> MTMPNGSGGLDPGAWLSHWVNQADLSSLAGRTEDEVRAYFENLVQADSGWGDASNTFFNLILGGFQNLSEFVTLIVQAVTGAPGGLTDLQAFLTERWGDLADAFQAVANLIDAIAGEVGSSLADAIAKLATFLTELSPLNAGMLFGLIGTNHLPLLSVSHIANINPELLVNAGFDSDVSVVDNPYWDWDGTVGRTAPLGAVKVVADGTIKDLLSGPDAIPVVEGQKLNVSAWLKYSGLVAGAGAGSIRLSGTAYSADGEVVAYPDFGGIPDGASGTSDWTQVTGQYVVPAGVTQFRLRLS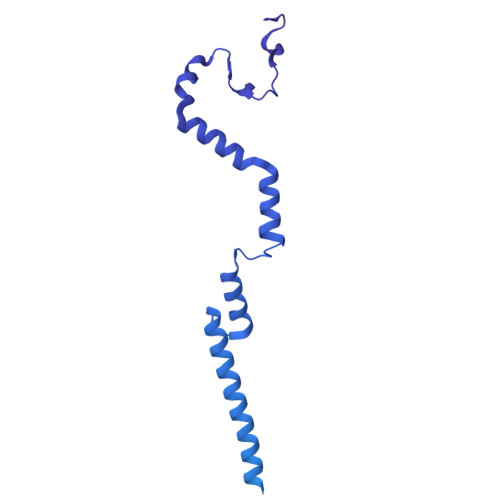VRENATGGTVWFDDCSVKKAGLLPQGLVDGLVQALSDLLTWLESLVDNVLSALGLDPIGTIVDKILDLADEFGDWLGATEDTAANLSNLLTKLLSDPASVIGPLAQSMITGLTGALGNLNTAINQIGDVLVGTVVTPINSAISNVIDWFNSLLNFQDTTTSNQINQQNFQIATLASGIKKQQWECRYSTAFVTFPEMFCDWGFALGGTTGAQSTGTAHTHTLNTDGLAALQIQILPAGYAIGGYIGISDTTIVDTIAMKMYKETSSAINNVYLEVFREDSTGALTSVGSVDVSGQLTTASDYVEATLPAGVIVNAGERYVVRMRNATTVGNRVGVSVMKELVGGRELSIRTETATDSNKTFYTPSEVLTAQGVSVIMPWAMMAAKNLATTDQSFSDDFNRSAMGGLWFLKSDTGTNQVGVSGGRAAFSGLTDGNQNALYIRPTAGDKQWVEATLYETGIAASGAREGLLMHANRDLSQVVYLGVNLNTAKIYTGPWNSLTERASVSTTGNDVLWQMYFDPATAAYTVLKNGQASGLTWTDSGSVVAHGPNYRFGGLRISRATFFNAGRIDNWTLKDWA>[2x]MMTMFEEVEVEAYVYPTEDIRKVKKAML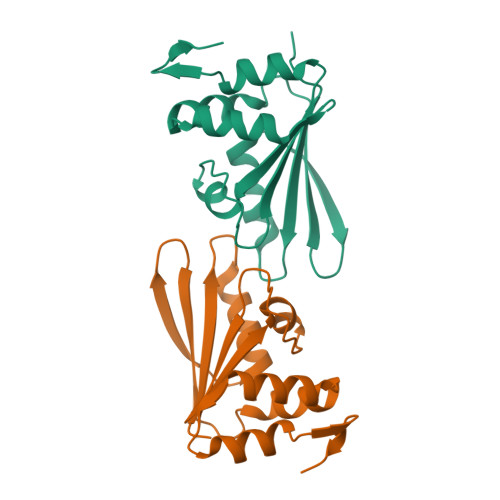NLIPGLQFEAFDKGEYVILVGRTKDKRALQRLYELFRGQQILDTARMMLEEGYFGEEIIIKVHKQVAYVGKVNFNEDSPLGPITITIRTKEPQKLMKWLAPRTKDGVPIE> GSHMGGLIYAVGGYNNSPDGHTHLSSLEAYNPSTDTWSPVAPMSVPRSGVGVAVIDGLIYAVGGYDGHTHLNSVEAYDPETDEWSLVAPMTTRRSGVGVAVLGGLIYAVGGYNNSPDGHTHLSSLEAYNPSTDTWSPVAPMSVPRSGVGVAVIDGLIYAVGGYDGHTHLNSVEAYDPETDEWSLVAPMTTRRSGVGVAVLGGLIYAVGGYNNSPDGHTHLSSLEAYNPSTD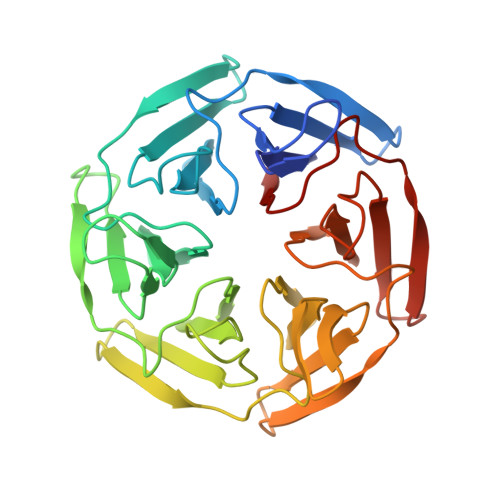TWSPVAPMSVPRSGVGVAVIDGLIYAVGGYDGHTHLNSVEAYDPETDEWSLVAPMTTRRSGVGVAVL> PVGAITTIEDPVLAKKVPETFPELKPGESRHTSDHMSIYKFMGRSHFLCTFTFNSNNKEYTFPITLSSTSNPPHGLPSTLRWFFNLFQLYRGPLDLTIIITGATDVDGMAWFTPVGLAVDTPWVEKESALQIDYKTALGAVRFNTRRTGNIQIRLPWYSYLYAVSGALDGLGDKTDSTFGLVSIQIANYNHSDEYLSFSCYLSVTEQSEFYFPRAPLNSNAMLST;> GASYFTSVDQSSVHTAEVGSHQIEPLKTSVDKPGSKKTQGEKFFLIHSARWLTTHALFHEVAKLDVVKLLYNEQFAVQGLLRYHTYARFGIEIQVQINPTPFQQGGLICAMVPGDQSYGSIASLTVYPHGLLNCNINNVVRIKVPFIYTRGAYHFKDPQYPVWELTIRVWSELNIGTGTSAYTSLNVLARFTDLELHGLTPLST;> MMRNETRVSTTENVVNLSNYEDARAKMSFALDQEDWKSDPSQGGGIKITHFTTWTSIPTLAAQFPFNASDSVGQQIKVIPVDPYFFQMTNTNPDQKCITALASICQMFCFWRGDLVFDFQ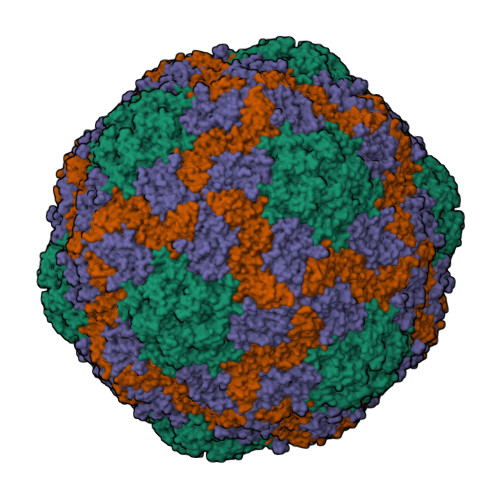VFPTKYHSGRLLFCFVPGNELIDVTGITLKQATTAPCAVMDIAGVQSTLRFRVPWISDTPYRVNRYTKEAHQKGEYTAIGKLIVYCYNRLTSPSNVAHHVRVNVYLSAINLECFAPLYHAMDVTTQ> GHHHHHHSKPDPVIPDPPIDPPPGTGKYTCPFAIWSLEEVYEPPTKNRPWPIYNAVELQPREFDVALKDLLGNTKWRDWDSRLSYTTFRGCRGNGYIDLDATYLATDQAMRDQKYDIREG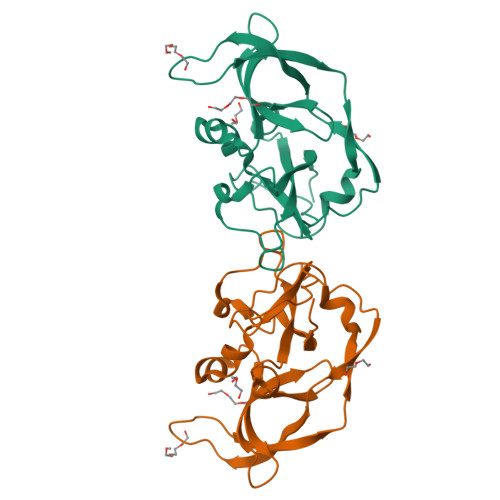KKPGAFGNIERFIYLKSINAYCSLSDIAAYHADGVIVGFWRDPSSGGAIPFDFTKFDKTKCPIQAVIVVPRA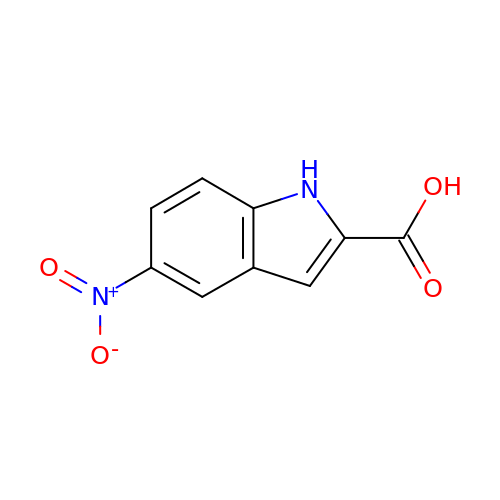5-nitro-1H-indole-2-carboxylic acid | C9 H6 N2 O4 | LHFOJSCXLFKDIR-UHFFFAOYSA-N> MEIDELTALGGLLHDIGKPVQRAGLYSGDHSTQGARFLRDLAENTGRAEYELLSLFSEFHHKGHMKNDELMIRRIKELSPERFGLTMEDVLNALWIVYEADNLASGEREEGQPQASRPLYSVFNPGKAYPWAELDFEKELPVPGDVFSIRSQDYRELVKRLWEELSKAKLRSDRLLPVLEKYLTFVSSVTSEGNIISLYDHMRMTSAIALAMLRAGCTAEDVRSGRCRKEKRFLLIEGDFSGIQDFIYRVSGKGTLKYLRARSAYLELIGWDVVLEILSRLGLTRANVVFNAGGHFMIIAQNT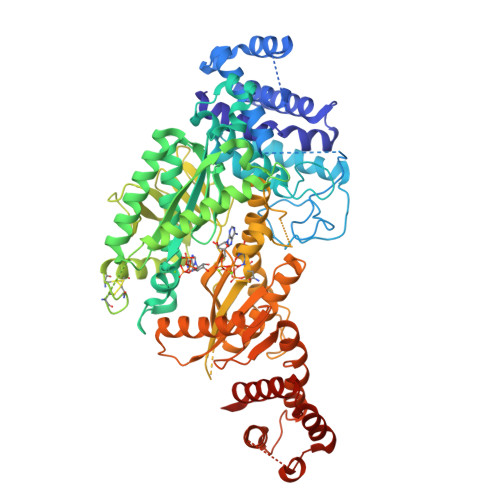PDAVKELEEIRAKAVEWLYREFESDLYLAIEWEPVSGREFGREGGKNLFAEARKRLKHKLTVRKLKRFGEIKGLFEHGHTERLAECPVCGRELPEGKLEPSASDPETKVCPTCNRLVSLGGNLPKLLGFGRTAKNDAGVLVEGPFSGFVPYLQGGRPVGEQILVKNTLNPGEIPESAQFVPYFVADYFKKDPKGGVAMEFGDYVKRASGIARLGVLRLDVDNLGQAFTHGFMEQGNGKFNTISRTAAFSRMLSLFFRQHINYVLARPKLRPITGDDPARPREATIIYSGGDDVFVVGAWDDVIEFGIELRERFHEFTQGKLTVSAGIGMFPDKYPISVMAREVGDLEDAAKSLPGKNGVALFDREFTFGWDELLSKVIEEKYRHIADYFSGNEERGMAFIYKLLELLAERDDRITKARWVYFLTRMRNPTGDTAPFQQFANRLHQWFQDPTDAKQLKTALHLYIYRTRKEESE>MAKIVLVLYDAGKHAADEEKLYGCTENKLGIANWLKDQGHELITTSDEEGGNSVLDQHIPDADIIITTPFHPAYITKERIDKAKKLKLVVVAGVGSDHIDLDYINQTGKKISVLEVTGSNVVSVAEHVVMTMLVLVRNFVPAHEQIINHDWEVAAIAKDAYDIEGKTIATIGAGRIGYRVLERLVPFNPKELLYYDYQALPKDAEEKVGARRVENIEELVAQADIVTVNAPLHAGTKGLINKELLSKFKKGAWLVNTARGAICVAE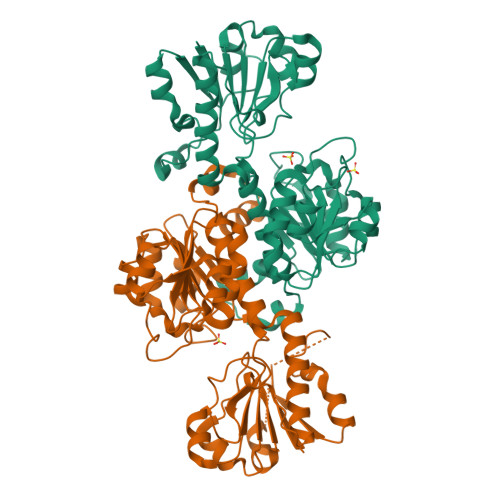DVAAALESGQLRGYGGDVWFPQPAPKDHPWRDMRNKYGAGNAMTPHYSGTTLDAQTRYAQGTKNILESFFTGKFDYRPQDIILLNGEYVTKAYGKHDKK[4x]> MSKLLMIGTGPVAIQLANICYLKSDYEIDMVGRASTSEKSKRLYQAYKKEKQFEVKIQNEAHQHLEGKFEINRLYKDVKNVKGEYETVVMACTADAYYDTLQQLSLETLQSVKHVILISPTFGSQMIVEQFMSKFSQDIEVISFSTYLGDTRIVDKEAPNHVLTTGVKKKLYMGSTHSNSTMCQRISALAEQLKIQLEVVESPLHAETRNSSLYVHPPLFMNDFSLKAIFEGTDVPVYVYKLFPEGPITMTLIREMRLMWKEMMAILQAFRVPSVNLLQFMVKENYPVRPETLDEGDIEHFEILPDILQEYLLYVRYTAILIDPFSQPDENGHYFDFSAVPFKQVYKNEQDVVQIPRMPSEDYYRTAMIQHIGKMLGIKTPMIDQFLTRYEASCQAYKDMHQDQQLSSQFNTNLFEGDKALVTKFLEINRTLSKGELNSKLEGKPIPNPLLGLDSTR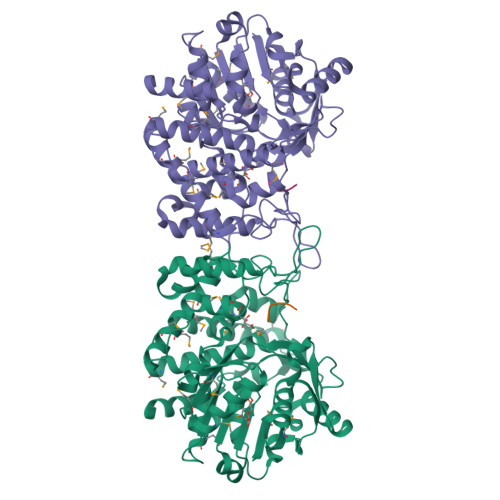TGHHHHHH;> AHHA> GPLGSPEFENKIEDIGQGAEIIKRTQDITSKRLAICQNIQFDFVKDKKYNKDALVVKMQGFISSRTTYSDLKKYPYIKRMIWPFQYNISLKTKDSN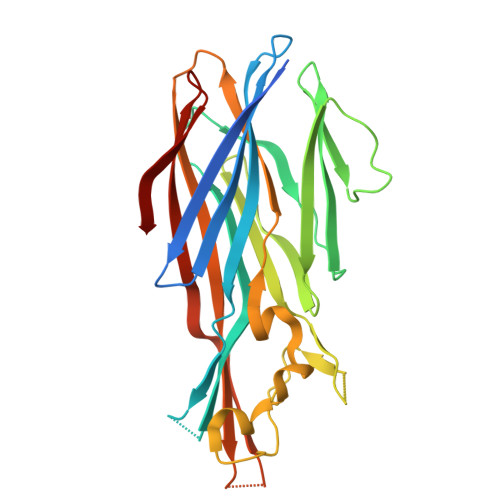VDLINYLPKNKIDSADVSQKLGYNIGGNFQSAPSIGGSGSFNYSKTISYNQKNYVTEVESQNSKGVKWGVKANSFVTPNGQVSAYDQYLFAQDPTGPAARDYFVPDNQLPPLIQSGFNPSFITTLSHEKGKGDKSEFEITYGRNMDATYAYVTRHRLAVDRKHDAFKNRNVTVKYEVNWKTHEVKIKSITPK>[2x]C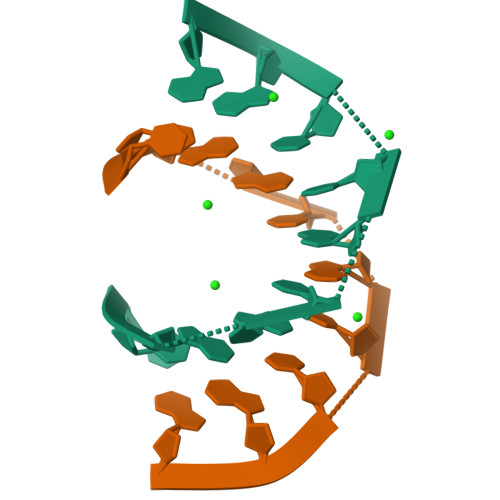CGGCGCCGG> MTEDRLSAEDKKFLEVERALKEAALNPLRHATEELFGDFLKMENITEICYNGNKVVWVLKNNGEWQPFDVRDRKAFSLSRLMHFARCCASFKKKTIDNYENPILSSNLANGERVQIVLSPVTVNDETISISIRIPSKTTYPHSFFEEQGFYNLLDNKEQAISAIKDGIAIGKNVIVCGGTGSGKTTYIKSIMEFIPKEERIISIEDTEEIVFKHHKNYTQLFFGGNITSADCLKSCLRMRPDRIILGELRSSEAYDFYNVLCSGHKGTLTTLHAGSSEEA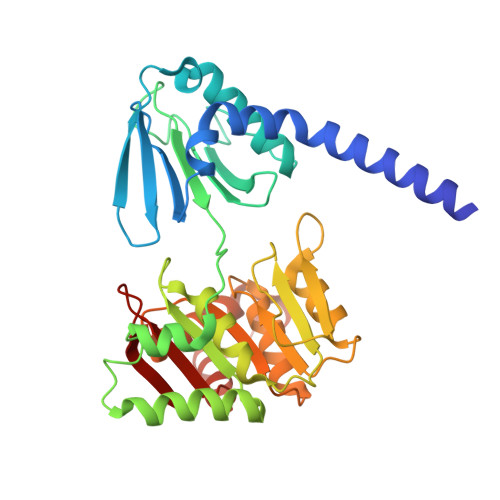FIRLANMSSSNSAARNIKFESLIEGFKDLIDMIVHINHHKQCDEFYIKHR> MATYDAKLRVWRGDDTGGELHDYTVEVNDGEVVLDIIHRLQATQTPDLAVRWNCKAGKCGSCSAEINGRPRLMCMTRMSTFGEDEVVTVTPLRTFPVMRDLVTDVSFNYEKARQIPSFTPPKDLQPGEYRMQQEDVNRSQEFRKCIECFLCQNVCHVVRDHEENKENFAGPRFHMRIAELDMHPLDTVDRKEMAQDEFGLGYCNITKCCTEVCPEHIKITDNALIPMKERVADRKYDP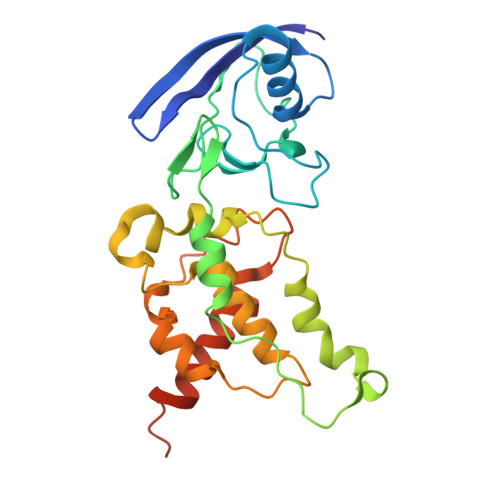IVWLGNKLFRR5-fluoro-1-[3-C-(hydroxymethyl)-beta-D-glucopyranosyl]pyrimidine-2,4(1H,3H)-dione | 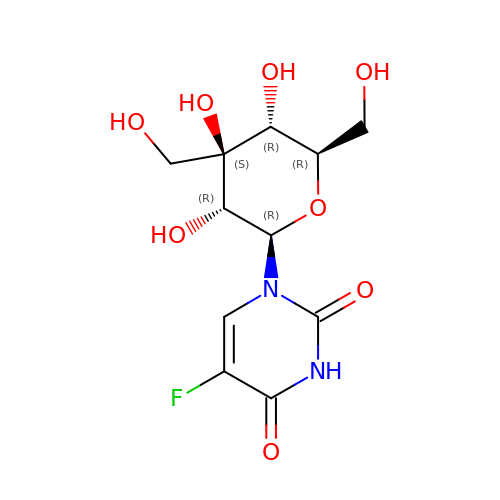C11 H15 F N2 O8 | ASRLDHHNHXDEKP-RZBPYSQRSA-N OGA is the unique enzyme responsible for O-GlcNAc hydrolysis from a large number of cytoplasmic and nuclear proteins. Recently, our group and others have independently identified crystallizable constructs of OGA that comprise the catalytic domain and stalk domain, and published the apo form structures and enzyme complexes with active site inhibitors. These reports consistently showed that OGA formed an unusual arm-in-arm homodimer, where the catalytic domain of one monomer covered by the stalk domain of the sister monomer to create a potential substrate-binding cleft. Exploiting our previously reported construct of OGAcryst (residues 60–704 with the unstructured insert residues 401–552 replaced by a glycine–serine (GS) linker), we solved the structures of a mutant OGAcryst-D175N (catalytically impaired but retaining the ability to bind substrate) in apo form and in complex with each of four synthetic glycopeptides.

A structural overlay of OGAcryst-D175N in the substrate-free and substrate-bound states illustrated that substrate binding did not induce any changes in the dimeric structure of OGA.

>[2x]HFLCGVVEGFYGRPWVMEQRKELFRRLQKWELNTYLYAPKDDYKHRMFWREMYSVEEAEQLMTLISAAREYEIEFIYAISPGLDITFSNPKEVSTLKRKLDQVSQFGCRSFALLFDNIDHNMCAADKEVFSSFAHAQVSITNEIYQYLGEPETFLFCPTEYCGTFCYPNVSQSPYLRTVGEKLLPGIEVLWTGPKVVSKEIPVESIEEVSKIIKRAPVIWDNIHANDYDQKRLFLGPYKGRSTELIPRLKGVLTNPNCEFEANYVAIHTLATWYKSNMNGVRKDVVMTDSEDSTVSIQIKLENEGSDEDIETDVLYSPQMALKLALTEWLQEFGVPHQYSSRGGGGSGGGGSVTLEDLQLLADLFYLPYEHGPKGAQMLREFQWLRANSSVVSVNCKGKDSEKIEEWRSRAAKFEEMCGLVMGMFTRLSNCANRTILYDMYSYVWDIKSIMSMVKSFVQWLGCRSHSSAQFLIGDQEPWAFRGGLAGEFQRLLPIDGANDLFFQ The androgen receptor (AR) is the cellular mediator of the actions of the hormone 5-α dihydrotestosterone (DHT). Androgen binding to AR leads to activation of genes involved in the development and maintenance of the male reproductive system and other tissues such as bone and muscle. AR is distinguished from other nuclear receptors in that after hormone binding, it preferentially responds to a specialized set of coactivators bearing aromatic-rich motifs, while responding poorly to coactivators bearing the leucine-rich “NR box” motifs favored by other nuclear receptors. Structures of AR in complex with FxxLF, LxxLL, FxxLW, WxxLF, WxxVW, FxxFF, and FxxYF motifs reveal a changing surface of the AR coactivator binding interface that permits accommodation of both AR-specific aromatic-rich motifs and canonical leucine-rich motifs.

To understand how the AR AF-2 accommodates tryptophan residues, structures of AR in complex with peptides containing tryptophan substitutions at the +1 or +5 position, or both, were determined. In FxxLW and WxxVW, the −2 serine forms a bidentate hydrogen-bonding interaction, making hydrogen bonds to both Glu897 and the backbone amide group of the +2 residue. However, the presence of a hydrogen-bonding partner on the indole side chain enables an additional polar interaction not seen in the phenylalanine-rich motifs between the indole nitrogen and Gln738. Unexpectedly, this additional interaction in the +1 pocket does not occur with Trp+1 of WxxVW. While similarly distanced to make the same interaction, the plane of the indole ring is rotated about 20° relative to that of WxxLF, causing it to be at a poor angle for strong hydrogen bonding to Gln738. Trp+5 of WxxVW is bound similarly to phenylalanine residues at the same position. Only the six-membered ring of the indole group is fully buried in the pocket. The five-membered ring of the indole side chain sticks out, solvent exposed.

> GSPGISGGGGGSHIEGYECQPIFLNVLEAIEPGVVCAGHDNNQPDSFAALLSSLNELGERQLVHVVKWAKALPGFRNLHVDDQMAVIQYSWMGLMVFAMGWRSFTNVNSRMLYFAPDLVFNEYRMHKSRMYSQCVRMRHLSQEFGWLQITPQEFLCMKALLLFSIIPVDGLKNQKFFDELRMNYIKELDRIIACKRKNPTSCSRRFYQLTKLLDSVQPIARELHQFTFDLLIKSHMVSVDFPEMMAEIISVQVPKILSGKVKPIYFHTQ;> SRWAEVWDDNSKVSR>[3x]GTDERVYESIGQYGGETVKIVRIEKARDIPLGATVRNEMDSVIISRIVKGGAAEKSGLLHEGDEVLEINGIEIRGKDVNEVFDLLSDMHGTLTFVLIPSQ;>NLNSSRVPDLLV[2x]

The C-terminus of the severe acute respiratory syndrome coronavirus 2 (SARS-CoV-2) protein E contains a PBM (PDZ-binding motif) targeting PDZ (PSD-95/Dlg/ZO-1) domains, which is identical to the PBM of SARS-CoV. Targeting multiple cellular PDZ (PSD-95/Dlg/ZO-1)-containing proteins through short linear PDZ-binding motifs (PBMs) is a common strategy used by viruses to facilitate their viral replication and dissemination to new hosts. PBMs are mainly located at the C-terminus of target proteins and interact directly with PDZ domains. We solved three crystal structures of complexes between human LNX2, MLLT4, and MPP5 PDZs and SARS-CoV-2 E PBM highlighting its binding preferences for several cellular targets.

As a key component of the Crumbs complex that controls the apical–basal polarity and TJ formation, MPP5 may contribute to the lung epithelium breakdown observed in patients infected by SARS-CoV. The crystal structure of the MPP5-PDZ in complex with SARS-CoV-2-E-PBM was solved at a resolution of 2.80 Å. There are three MPP5-PDZs per asymmetric unit. Each domain adopts a compact globular PDZ fold, and an electron density was observed for the last five residues of the peptide in two MPP5-PDZs present in the asymmetric unit. As for MLLT4, the E PBM conventionally binds to the MPP5-PDZ. The C-terminal carboxylate of the Val at position 0 of the PBM forms two hydrogen bonds: one with the amide proton of Leu 267 and one with Gly 268 of the “GLGF” loop of MPP5-PDZ. In addition, the amide and carbonyl groups of Leu at position -2 form hydrogen bonds with the carbonyl and amide proton of valine 271, respectively. Interestingly, as for MLLT4, a hydrogen bond is also formed between the carboxyl at the end of the side chain of Asp at position -3 of the PBM and the hydroxyl group of Ser 281 of the β3 strand. The alternative hydrogen bond with Ser 281 identified in our structure was previously reported in the complex formed by MPP5-PDZ and the PBM peptide of Crumbs. Furthermore, the side chain of Phe 318 in α2 helix, which prevents access to the binding groove in the unbound form, is located out of the binding groove in our structure allowing SARS-CoV-2-E-PBM peptide binding as previously stated for MPP5-PDZ in complex with SARS-CoV-1 E and SARS-CoV-2 E PBMs, as well as for Crumbs peptides.>MGHHHHHHPFRATGDGLFIMNEGNFQYGNATLSYYDPETKKVENEIFYRANAMKLGDVAQSMIVRDTIGWVVVNNSHVIFAISTNTFKEVGRITGLTSPRYIHFISDEKAYITQIWDYRIFIVNPKTYQITGYIECPDMTMETGSTEQMVQYGKYVYVNCWSYQNRILKIDTTTDKVVDQLTVGIQPTSLVMDKNFKMWTITDGGYKGSPYGYEEPSLYRIDAETFKIEKQFKFQLGDAPSEVQLNGAGDELYWINKDIWRMSVDEERVPVRPFLKYRDTKYYGLTVSPKNGDVYVADAIDYQQQGMIYRYTEDGELVDEFYVGIIPGAFCWK[4x]

Contrasting with Enterobacteria, members of the dominant genus Bacteroides often encode several BtuB vitamin B12 outer membrane transporters together with a conserved array of surface-exposed B12-binding lipoproteins. Here we show that the BtuB transporters from Bacteroides thetaiotaomicron form stable, pedal bin-like complexes with surface-exposed BtuG lipoprotein lids, which bind B12 with high affinities. Closing of the BtuG lid following B12 capture causes destabilisation of the bound B12 by a conserved BtuB extracellular loop, causing translocation of the vitamin to BtuB and subsequent transport. We propose that TonB-dependent, lipoprotein-assisted small molecule uptake is a general feature of Bacteroides spp. that is important for the success of this genus in colonising the human gut.

To compare CNCbl binding to BtuB3G3 and BtuG3 alone, we also determined the crystal structure of BtuB3-CNCbl to a resolution of 2.6 Å. A superposition of BtuG3-CNCbl onto BtuB3G3-CNCbl (state 1) has a Cα RMSD of ~0.6 Å, demonstrating that CNCbl binding to BtuG3 and BtuB3G3 is virtually identical. Moreover, BtuG2 and BtuG3 share 80% sequence identity, and a superposition of both structures bound to CNCbl shows that residues binding the ligand are the same and the overall structure is identical (Cα RMSD ~ 0.4 Å). Thus, we conclude that CNCbl binding by BtuG2 and BtuG3 is the same.>[2x]GRKERERLEEKLEDANERIAELVKLEERQRIARDLHDTLGQKLSLIGLKSDLARKLIYKDPEQAARELKSVQQTA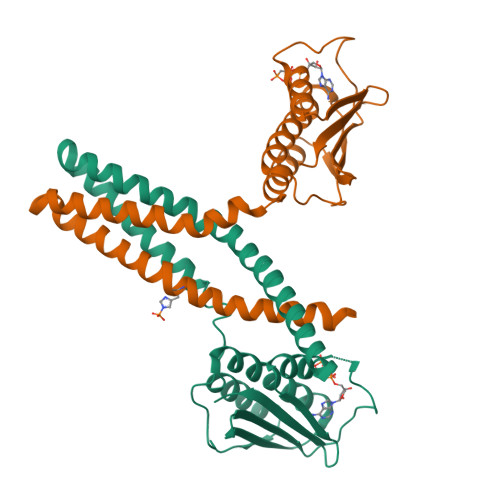RTSLNEVRKIVSSMKGIRLKDELINIKQILEAADIMFIYEEEKWPENISLLNENILSMCLKEAVTNVVKHSQAKTCRVDIQQLWKEVVITVSDDGTFKGEENSFSKGHGLLGMRERLEFANGSLHIDTENGTKLTMAIPNNSK> LPTDTTTFKRIFLKRMPSIRESLKERGVDMARLGPEWSQPMKRLTLGNTTSSVILTNYMDTQYYGEIGIGTPPQTFKVVFDTGSSNVWVPSSKCSRLYTACVYHKLFDASDSSSYKHNGTELTLRYSTGTVSGFLSQDIITVGGITVTQMFGEVTEMPALPFMLAEFDGVVGMGFIEQAIGRVTPIFDNIISQGVLKEDVFSFYYNRDSENSQSLGGQIVLGGSDPQHYEGNFHYINLIKTGVWQIQMKGVSVGSSTLLCEDGCLALVDTGASYISGSTSSIEKLMEALGAKKRLFDYVVKCNEGPTL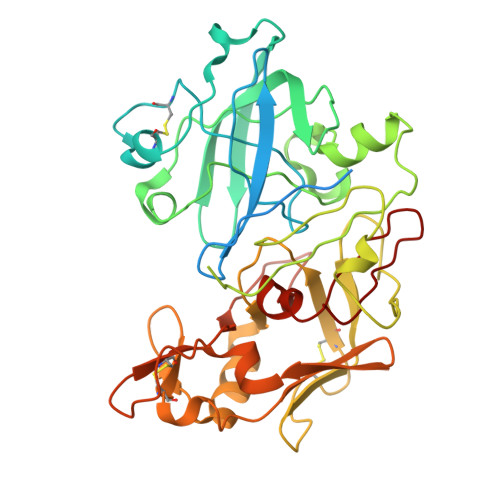PDISFHLGGKEYTLTSADYVFQESYSSKKLCTLAIHAMDIPPPTGPTWALGATFIRKFYTEFDRRNNRIGFALAR> QVQQEPSAETSEGTGINITCSHPSIQAYSIQWYRQLPGRGPAFLVSAVKGSKEVPDPEGRLSVSADSRSSALWLARPRLGDAAVYYCAVRG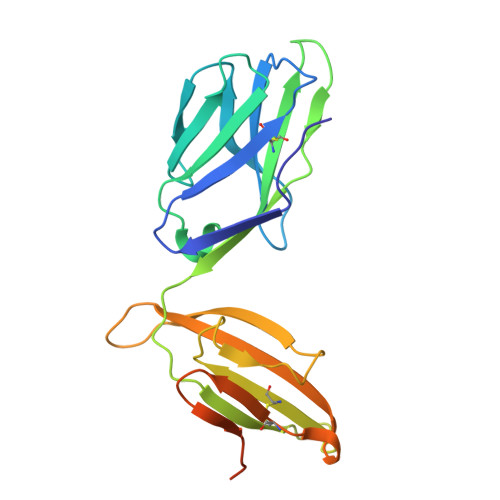SSYTKLTFGTGTRLSVQPHITPSPSVYRLTSEDNKNLEMCLITDYSPEKLDLSSVDSKTETVVEVATSENKHEASYLSTYWAKKDEMQCGAKHEGFGILKGDDPEAGASTVCITGMSLLFKTDENLN>MIELSLAEALFLILFTGVISMLISRRTGISYVPIFILTGLVIGPLLKLIPRDLAHEIFDFVRVFGLVIILFTEGHNLSWRLLKKNMPTIVTLDTIGLILTALIAGFIFKVVFNSSFLLGFLFGAIIGATDPATLIPLFRQYRVKQDIETVIVTESIFNDPLGIVLTLIAISMLVPGYGGGIFSTLSEKLGIYAGGVIYFLYNVSVSISLGIFLGILGYKFIKRTGIFDFPEIEAFSLSLAFLGFFIGERLDASGYLVATVTGIVLGNYKLLKPRENIRILKRLQRAIEKEVHFNDTLAALATIFIFVLLGAEMNLEVIWSNLGKGLLVALGVMILARPLATLPLLKWWNFREYLFIALEGPRGVVPSALASLPLSLALKYKSPLLTVHWGEIIMATVVITVLTSVIVETLWIPILKDKLDVG[2x]

H5 and H12 in the 6-helix bundle are discontinuous. dimer indicates clusters of charged residues on both sides of the membrane. transported by PaNhaP, K+ is not. structure thus serves as an excellent model for the membrane part of NHE1.

The structure was solved at 3.15  Å by SeMet-SAD. The structure was solved by SAD. ethanolamine (PE), carried over from the E. coli expression host. Six ion bridges that lock the two protomers together at pH 8 break at pH 4.>[6x]GA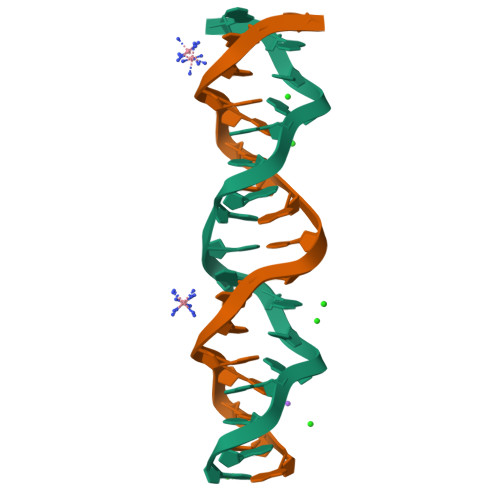CGACGACGACGACGA>[2x]MELGAGGVVFNAKREV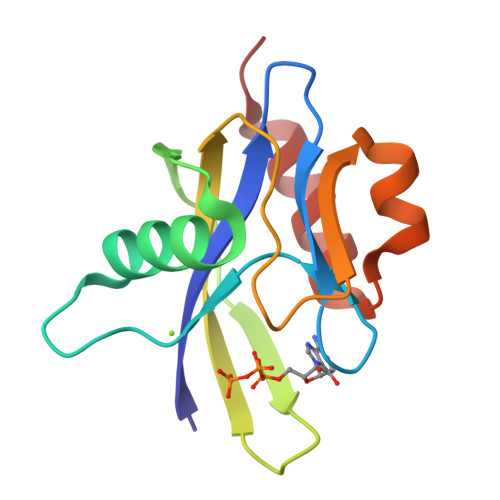LLLRDRMGFWVFPKGHPEPGESLEEAAVREVWEQTGVRAEVLLPLYPTRYVNPKGVEREVHWFLMRGEGAPRLEEGMTGAGWFSPEEARALLAFPEDLGLLEVALERLPL> APAAVDWR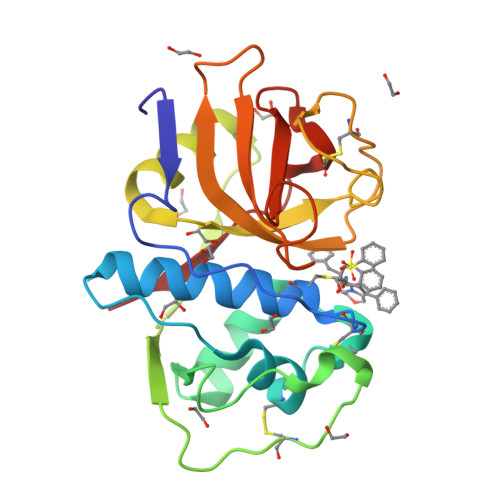EKGAVTPVKDQGQCGSCWAFSTIGNIEGQWQVAGNPLVSLSEQMLVSCDTIDFGCGGGLMDNAFNWIVNSNGGNVFTEASYPYVSGNGEQPQCQMNGHEIGAAITDHVDLPQDEDAIAAYLAENGPLAIAVDATSFMDYNGGILTSCTSEQLDHGVLLVGYNDASNPPYWIIKNSWSNMWGEDGYIRIEKGTNQCLMNQAVSSAVVG>SKPKQPPDASPANLLTSLVRAHLDSGPSTAKLDYSKFQELVLPHFGKEDAGDVQQFYDLLSGSLE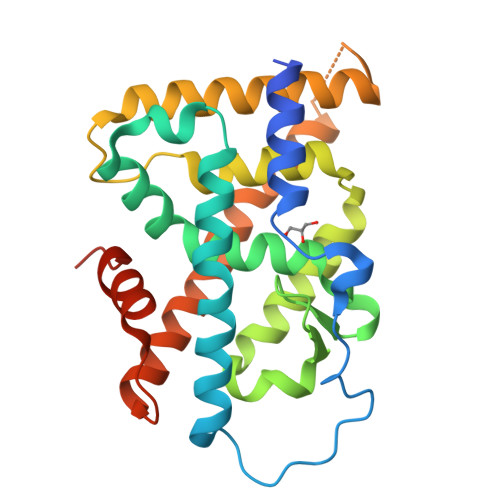VIRKWAEKIPGFAELSPADQDLLLESAFLELFIWRLAYRSKPGEGKLIFCSGLVLHRLQCARGFGDWIDSILAFSRSLHSLLVDVPAFACLSALVLITDRHGLQEPRRVEELQNRIASCLKEHVAAVAGEPQPASCLSRLLGKLPELRTLCTQGLQRIFYLKLEDLVPPPPIIDKIFMDTLPFLEHHHHHH[2x]> MRQASRLALSIRQAGNVEAASAVPAMTRQFSAPGSHEHHETPLSKVMPTVVSIPRKVACLALGATKKVVCGLASSGPSQNLVSTFANKVIVEENLVNVAEIDVPFWSYWLSSAGFTSKDAFVKFAEAVKPKVAALSTSDI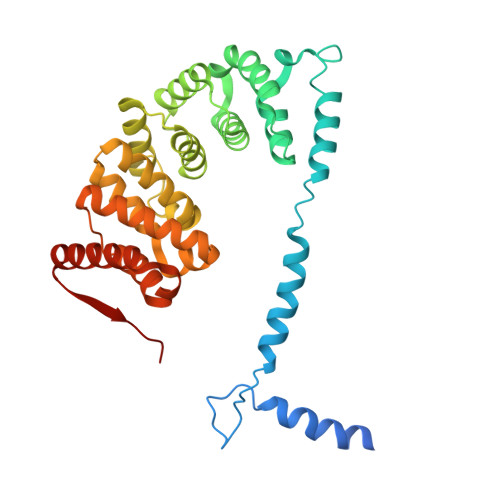TNLTVAFKRANYYDKDLFTGIEANVSANFTKFETEQLLQIVATFDAFNHSSVAFLDDVADSITYCNHYLAPVRAGADELATLLTYYAKNGHERADLLATVARGFSEVSLGKLSAAQRKDTVLSALKAFQTFGFYPESIEAVIGAALVSPAEYSAEELKEVEAVKVAAENALGGEFVLIQEGAHGH> MHGRL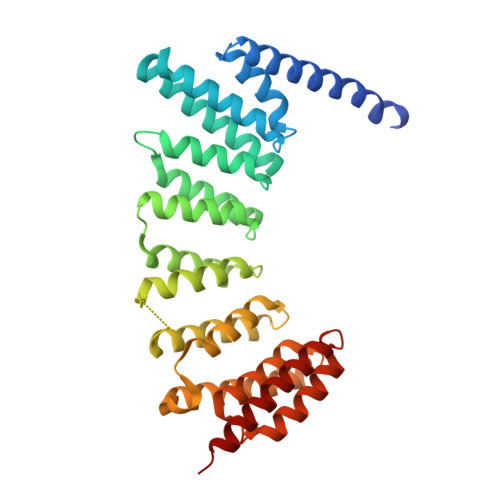KVKTSEEQAEAKRLEREQKLKLYQSATQAVFQKRQAGELDESVLELTSQILGANPDFATLWNCRREVLQHLETEKSPEESAALVKAELGFLESCLRVNPKSYGTWHHRCWLLSRLPEPNWARELELCARFLEADERNFHCWDYRRFVAAQAAVAPAEELAFTDSLITRNFSNYSSWHYRSCLLPQLHPQPDSGPQGRLPENVLLKELELVQNAFFTDPNDQSAWFYHRWLLGAGSGRCELSVEKSTVLQSELESCKELQELEPENKWCLLTIILLMRALDPLLYEKETLQYFSTLKAVDPMRAAYLDDLRSKFLLENSVLKMEYA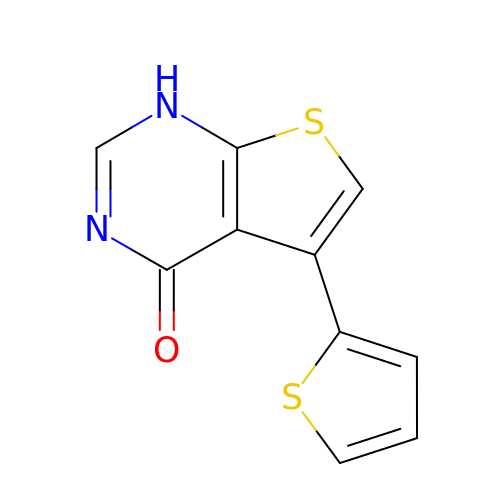5-(thiophen-2-yl)thieno[2,3-d]pyrimidin-4(1H)-one | C10 H6 N2 O S2 | LFUBTAOTPHKKOS-UHFFFAOYSA-N~{N}-[(5~{S})-6-azanyl-5-[[2,3-bis(oxidanyl)phenyl]carbonylamino]-6-oxidanylidene-hexyl]-2,3-bis(oxidanyl)benzamide | C45 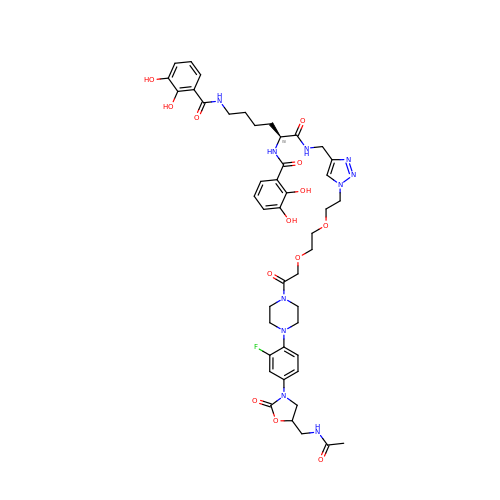H55 F N10 O13 | MCQYNUWYVGRUPW-IKAUJVHPSA-N>[2x]STAGKVIKCKAAVLWEQKKPFSIEEVEVAPPKAHEVRIKMVAAGICRSDDHVVSGTLVAPLPVIAGHEAAGIVESIGEGVTTVRPGDKVIPLFIPQCGKCSVCKHP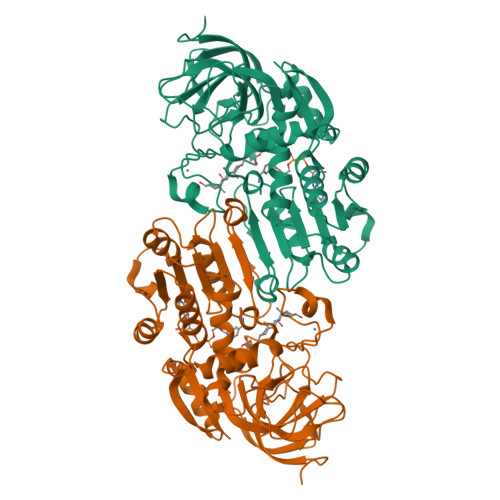EGNLCLKNLSMPRGTMQDGTSRFTCRGKPIHHFLGTSTFSQYTVVDEISVAKIDAASPLEKVCLVGCGFSTGYGSAVKVAKVTQGSTCAVFGLGGVGLSVIMGCKAAGAARIIGVDINKDKFAKAKEVGATECVNPQDYKKPIQEVLTEMSNGGVDFSFEVIGRLDTMVAALSCCQEAYGVSVIVGVPPDSQNLSMNPMLLLSGRTWKGAIFGGFKSKDSVPKLVADFMAKKFALDPLITHVLPFEKINEGFDLLRSGKSIRTILTF> MQTLKELIASNPDDLTTELKRAFRPLTPHIAIDGNELDALTILVNLTDKTDDQKDLLDRAKCKQKLRDEKWWASCINCVNYRQSHNPKFPDIRSEGVIRTQALGELPSFLLSSSKIPPYHWSYSHDSKYVNKSAFLTNEFCWDGEISCLGELLKDADHPLWNTLKKLGCSQKTCKAMAKQLADITLTTINVTLAPNYLTQISLPDSDTSYISLSPVASLSMQSHFHQRLQDENRHSAITRFSRTTNMGVTAMTCGGAFRMLKSGAKFSSPPHHRLNSKRSWLTSEHVQSLKQYQRLNKSLIPENSRIALRRKYKIELQNMVRSWFAMQDHTLDSNILIQHLNHDLSYLGATKRFAYDPAMTKLFTELLKRELSNSINNGEQHTNGSFLVLPNIRVCGATALSSPVTVGIPSLTAFFGFVHAFERNINRTTSSFRVESFAICVHQLHVEKRGLTAEFVEKGDGTISAPATRDDWQCDVVFSLILNTNFAQHIDQDTLVTSLPKRLARGSAKIAIDDFKHINSFSTLETAIESLPIEAGRWLSLYAQSNNNLSDLLAAMTEDHQLMASCVGYHLLEEPKDKPNSLRGYKHAIAECIIGLINSITFSSETDPNTIFWSLKNYQNYLVVQPRSINDETTDK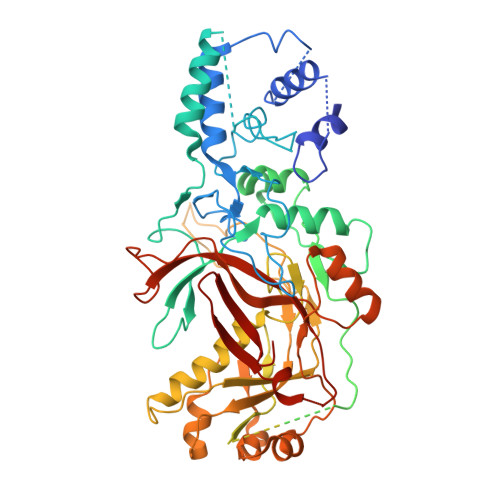SSL> MVFEFLFYNQQHKTRNGYFINHDNLMLASLEERKKLIFYFIANQVPEKLDPVDRVKFNEELSDNLSTKARLIGSLTGLIGLVGFPYISTRIYSRPVLNIGLSL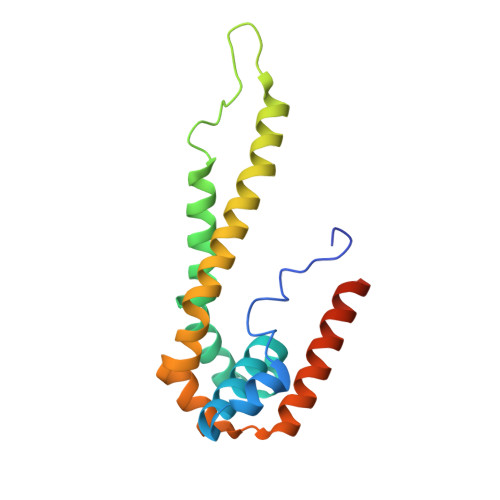LICPFLYYVGNQLTYSVWEPKFIANNNTVCELSKKYNFTVFDFAQAKKEAHLKALRTELVSDNLLYSPGI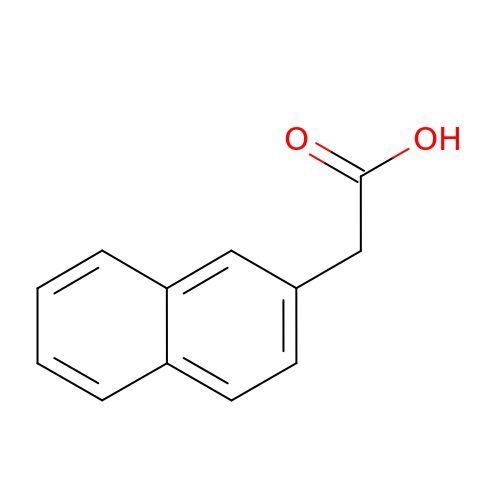2-naphthalen-2-ylethanoic acid | C12 H10 O2 | VIBOGIYPPWLDTI-UHFFFAOYSA-N>MIRTGKQYLESLNDGRNVWVGNEKIDNVATHPKTRDYAQRHADFYDLHHRPDLQDVMTFVDKDGERRTMQWFGHYDKEQLRRKRKYHETIMREMAGASFPRTPDVNNYVLQTYIDDPSPWETQTIGAEGKVKAKNIVDFVNFAKKHDLNCAPQFVDPQMDRSNPDAQQRSPGLRVIEKNDKGIVVSGVKAIGTGVAFADWIHIGVFFRPGIPGDQIIFAATPVNTPGVTIVCRESVVKEDPIEHPLASQGDELDGMTVFDNVFIPWSHVFHLGNPEHAKLYPQRVFDWLHYHALIRQSVRAELMAGLAILITEHIGTNKIPAVQTRVAKLIGFHQAMLAHIVASEELGFHTPGGAYKPNILIYDFGRALYLENFSQMIYELVDLSGRSALIFASEDQWNDEALNGWFERMNNGPVGQPHDRVKIGRVIRDLFLTDWGNRLFVFENFNGTPLQAIRMLTMQRAEFSAAGPYGTLARKVCGIELTEGHDSEYKATAGYAQALDSARHQEKLALSGTMTV[4x]

The first enzyme in the 2,4,6-TCP degradation pathway of C. necator JMP134, 2,4,6-TCP 4-monooxygenase (TcpA), is responsible for the conversion of 2,4,6-TCP to 6-chloro-2-hydroxy-p-hydroquinone (6-CHQ). TcpA converts 2,4,6-TCP to 2,6-DiCBQ by oxidative reaction, followed by removing another chlorine by hydrolytic reaction, producing 6-chloro-2-hydroxy-p-hydroquinone. 2,4,6-Trichlorophenol-4-monoxygenase is a unique enzyme that catalyzes the sequential dechlorination of 2,4,6-TCP to 6,-CHQ in a single active site through both oxydative and hydrolytic reactions.

Recombinant TcpA from C. necator JMP134 was crystallized in the space group C2, with cell dimensions of a = 107.07 Å, b = 180.05 Å, c = 110.20 Å, β = 97.87 and there were four TcpA molecules in the asymmetric unit. The individual TcpA molecules consisted of fourteen β-strands and eighteen α-helices and could be divided into three sequential segments based on their constituent secondary structural elements. All the nine β-strands in the second segment, β4-β12, were arranged in such a way to appear almost like a β-barrel. Another noticeable structural feature was that three long α-helices, α10, α11 and α12, and three short helices, α15, α16 and α17, which were all from the C-terminal segment, formed a sizeable helix bundle together with two short α-helices from the first segment, α4 and α5. Applying a two-fold symmetry operation to one of the two dimers in the asymmetric unit generates one tightly associated tetramer in a non-crystallographic D2 symmetric assembly. The tetrameric nature of TcpA in solution was confirmed by the elution profile and molecular weight estimates from a multi-angle laser light scattering (MALLS) experiment. The observed tetramer interface had an extensive network of inter-subunit interaction among the C-terminal α-helices. In the apo-structure of TcpA, a unique entry site and binding pocket for FADH2 were clearly distinguishable. The perimeter of the widely open entry site was made with three flexible loops: (i) between β4 and β5; (ii) between β7 and β8; and (iii) between α16 and α17. A structural alignment of both TcpA and TftD showed that the global structure of the two enzymes were quite similar with an r.m.s.d. of 0.78 between Cα atoms.>[2x]MKVMECQTYEELSQIAARITADTIKEKPDAVLGLATGGTPEGTYRQLIRLHQTENLSFQNITTVNLDEYAGLSSDDPNSYHFYMND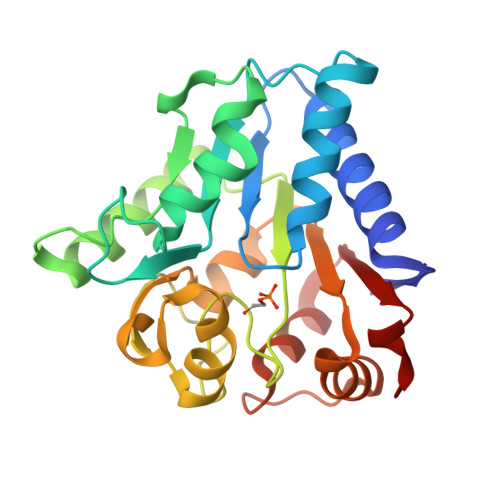RFFQHIDSKPSRHFIPNGNADDLEAECRRYEQLVDSLGDTDIQLLGIGRNGHIGFNEPGTSFKSRTHVVTLNEQTRQANARYFPSIDSVPKKALTMGIQTILSSKRILLLISGKSKAEAVRKLLEGNISEDFPASALHLHSDVTVLIDREAASLRP> MKLDIKKTFSNRSDRVKGIDFHPTEPWVLTTLYSGRVEIWNYETQVEVRSIQVTETPVRAGKFIARKNWIIVGSDDFRIRVFNYNTGEK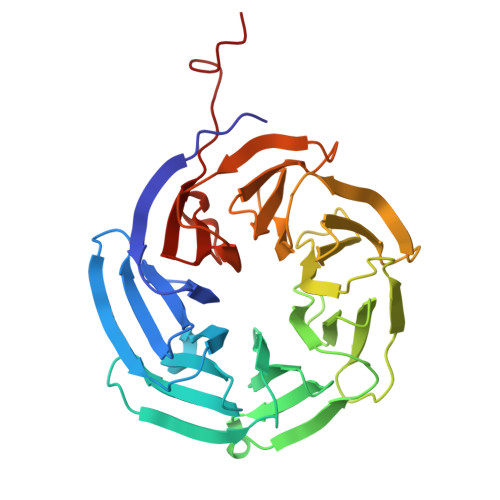VVDFEAHPDYIRSIAVHPTKPYVLSGSDDLTVKLWNWENNWALEQTFEGHEHFVMCVAFNPKDPSTFASGCLDRTVKVWSLGQSTPNFTLTTGQERGVNYVDYYPLPDKPYMITASDDLTIKIWDYQTKSCVATLEGHMSNVSFAVFHPTLPIIISGSEDGTLKIWNSSTYKVEKTLNVGLERSWCIATHPTGRKNYIASGFDNGFTVLSLGVIHNISSHED>[2x]MSLNSAAQAQSSDPVVIGCPAPLTGIVAADGIEFQRGIQMAADEINAVGGILGRPIELVFADTQSKGVDVVIQSAQRLIDRDNASALIAGYNLENGTALHDVAADAGVIAMHANTVAVHDEMVKSDPDRYWGTFQYDPPETLYGGGFLKFLKDIEDNGEFSRPNNKIAIITGPGIYSVNIANAIRDGAGEYGYDVSLFETVAIPVSDWGPTLAKLRADPPAVIVVTHFYPQ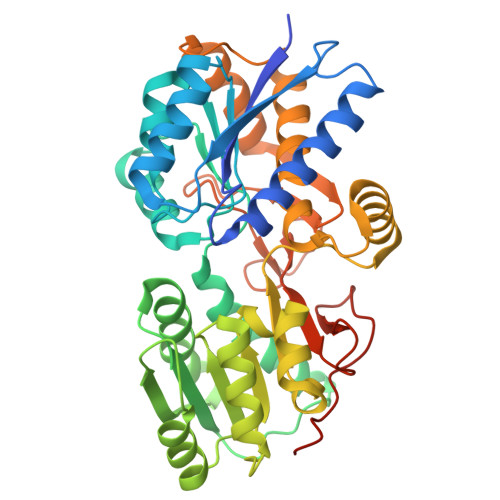DQALFMNQFMTDPTNSLVYLQYGASLAAFRDIAGDNSVGVTYATVLGTLQDEMGDAFAKAYKERYGDLSSTASGCQTYSALYAYSIAAALAGGPGAPYDDVQNKAVADRLRSLIFRGPVGTMRFHADTQSAWSYPTETNDPSLGMPHIFSQIFDKAEDGVLIAPAPYKKAGFKMPPWMKGEGHHHHHH> TYKFFE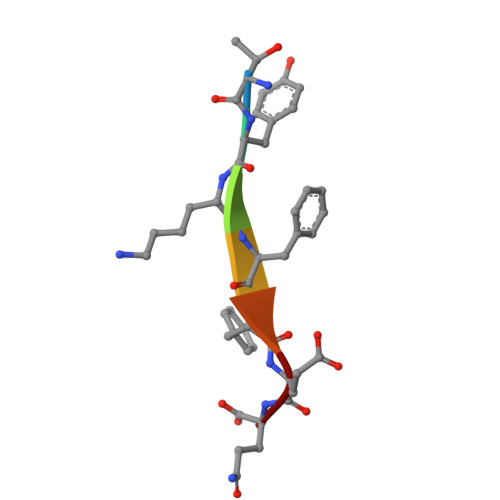Q> GSSMGSDEQRRELEEKIKWKLAELASKSEEERKEIKLRVIAYVLVQLEDLQKNLSDEQRRE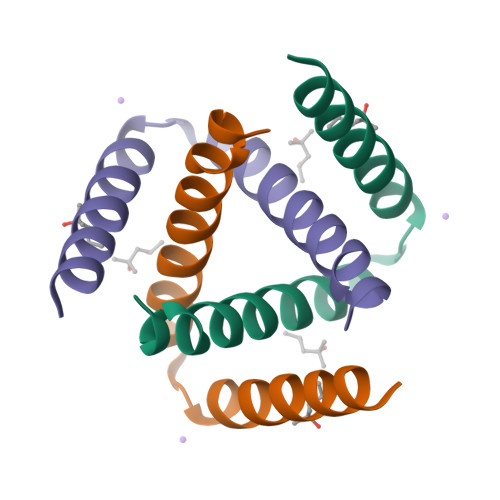LEEKIKWKLAELASKSEEERKEIKLRVIAYVLVQLEDLQKNLSDEQRRELEEKIKWKLAELASKSEEERKEIKLRVIAYVLVQLEDLQKNLS dodecyl 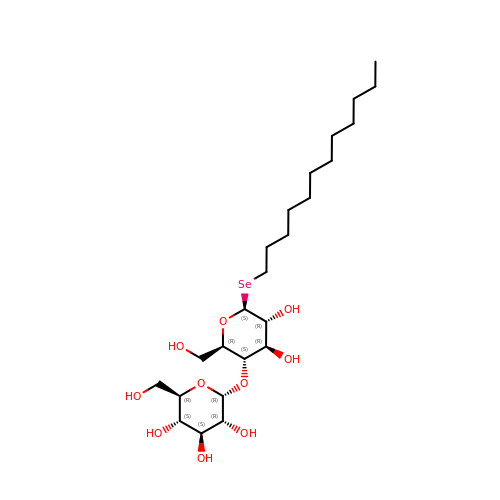4-O-alpha-D-glucopyranosyl-1-seleno-beta-D-glucopyranoside | C24 H46 O10 Se | MEIBWTYMLPEGMV-ALYNCGSASA-N> MQPQLSRPQTASNQVRKAVSGPWSGNAVHKAEKYFITSAKRDRDGKLQIELVPASGRRKLSPTPEMIRRLIDGEIEIYILTTQPDIAIDMNKEIIDMENRYVIDFDKRGVKWTMREIPVFYHEGKGLCVELHNKIYTLDQF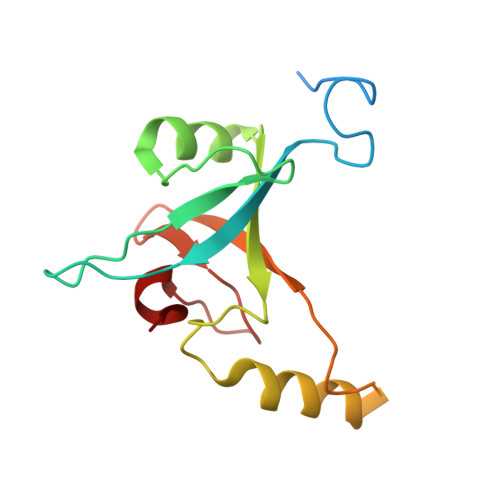FK> SQIPASEQETLVRPKPLLLKLLKSVGAQKDTYTMKEVL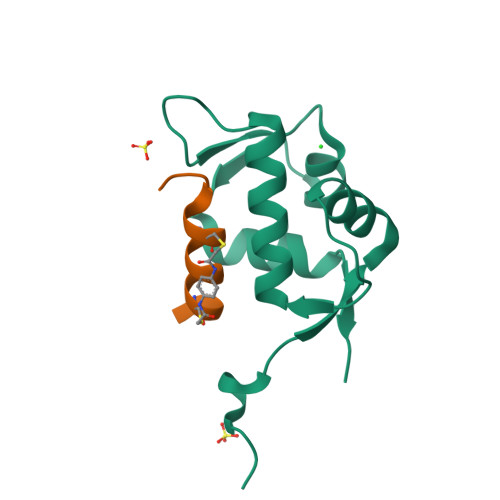FYLGQYIMTKRLYDEKQQHIVYCSNDLLGDLFGVPSFSVKEHRKIYTMIYRNLVVVN;> XDPAWYECLEAALLCQQVX>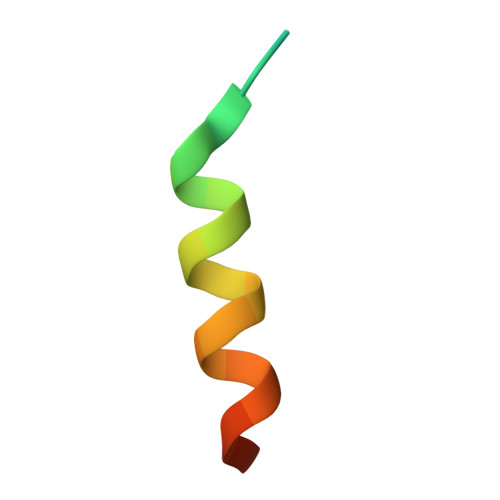 STSASEDIDFDDLSRRFEELKKKTW>[2x]LLVPKLTASVTDGAVGVTVDAPVSVTAADGVLAAVTMVNDNGRPVAGRLSPDGLRWSTTEQLGYNRRYTLNATALGLGGAATRQLTFQTSSPAHLTMPYVMPGDGEVVGVGEPVAIRFDENIADRGAAEKAIKITTNPPVEGAFYWLNNREVRWRPEHFWKPGTAVDVAVNTYGVDLGEGMFGEDNVQTHFTIGDEVIATADDNTKILTVRVNGEVVKSMPTSMGKDS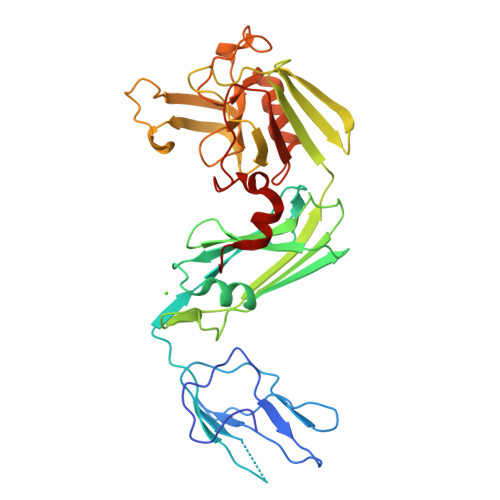TPTANGIYIVGSRYKHIIMDSSTYGVPVNSPNGYRTDVDWATQISYSGVFVHSAPWSVGAQGHTNTSHGCLNVSPSNAQWFYDHVKRGDIVEVVNTVGGTLPGIDGLGDWNIPWDQWRAGNAKA>[2x]GSQAANDAANKLFSLTIADLTANQN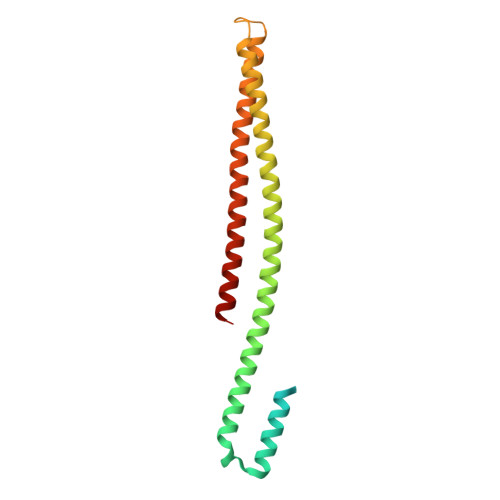INTTNAHSTSNILIPELKAPKSLNASSQLTLLIGNLIQILGEKSLTALTNKITAWKSQQQARQQKNLEFSDKINTLLSETEGLTRDYEKQINKLKNADSKIKDLENKINQIQTRLSELDPESPEKKKLSREEIQLTIKKDAAVKDRTLIEQKTLSIHSKLTDKSMQLEKEIDSFSA> EEEEEDAGLVAEAEAVAAGWMLDFLCLSLCRAFRDGRSEDFRRTRNSAEA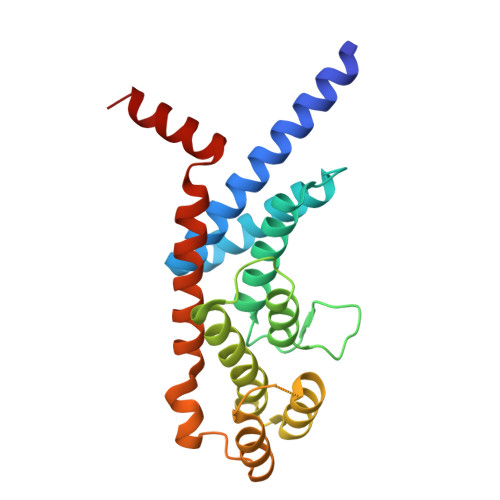IIHGLSSLTACQLRTIYICQFLTRIAAGKTLDAQFENDERITPLESALMIWGSIEKEHDKLHEEIQNLIKIQAIAVCMENGNFKEAEEVFERIFGDPNSHMPFKSKLLMIISQKDTFHSFFQHFSYNHMMEKIKSYVNYVLSEKSSTFLMKAAAKVVESKR> GPGS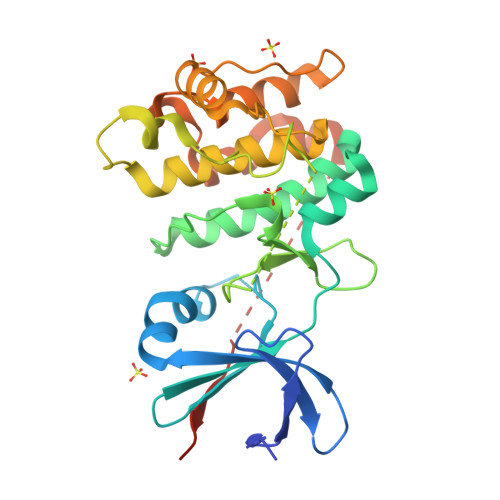APGPSRIADYLLLPLAEREHVSRALCIHTGRELRCKVFPIKHYQDKIRPYIQLPSHSNITGIVEVILGETKAYVFFEKDFGDMHSYVRSRKRLREEEAARLFKQIVSAVAHCHQSAIVLGDLKLRKFVFSTEERTQLRLESLEDTHIMKGEDDALSDKHGCPAYVSPEILNTTGTYSGKAADVWSLGVMLYTLLVGRYPFHDSDPSALFSKIRRGQFCIPEHISPKARCLIRSLLRREPSERLTAPEILLHPWFESVLEPGYIDSEIGTSDQIVPEYQEDSDISSFFS> MSLADFMEQRVQVITNDGRVVLGSLKGFDHTTNLILSDSFE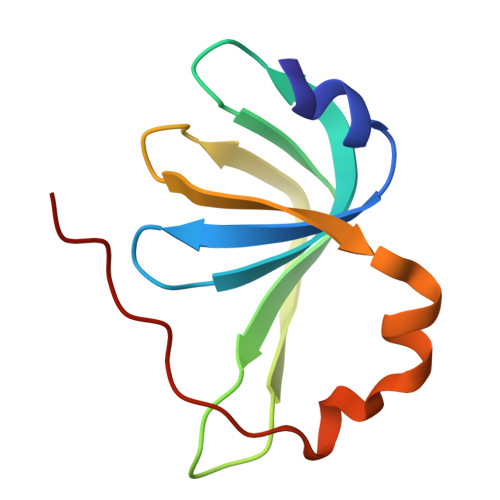RIISMDQDMETIPLGVYLLRGENVAMVGLVNEELDSEIEWTKIRGEAIPDVVH> MKTMRKQIYKKAYWLLLPFLPLALANTFLVKEDSKNVTAYTPFATPITDSKSDLVSLAQLDSSYQIADQTIHNTNLFVLFKSRDVKVKYESSGSNNISFDSTSQGEKPSYVVEFTNSTNIGIKWTMVKKYQLDVPNVSSDMNQVLKNLILEQPLTKYTLNSSLAKEKGKTQREVHLGSGQANQWTSQRNQHDLNNNPSPNASTGFKLTTGNAYRKLSESWPIYEPIDGTKQGKGKDSSGWSSTEENEAKNDAPSVSGGGSSSGTFNKYLNTKQALESIGILFDDQTPRNVITQLYYASTSKLAVTNNHIVVMGNSFLPSMWYWVVERSAQENASNKPTWFANTNLDWGEDKQKQ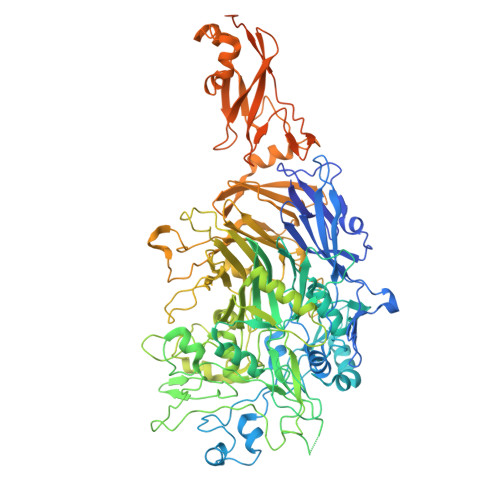FVENQLGYKETTSTNSHNFHSKSFTQPAYLISGIDSVNDQIIFSGFKAGSVGYDSSSSSSSSSSSSTKDQALAWSTTTSLDSKTGYKDLVTNDTGLNGPINGSFSIQDTFSFVVPYSGNHTNNGTTGPIKTAYPVKKDQKSTVKINSLINATPLNSYGDEGIGVFDALGLNYNFKSNQERLPSRTDQIFVYGIVSPNELRSAKSSADSTGSDTKVNWSNTQSRYLPVPYNYSEGIIDADGFKRPENRGASVTTFSGLKSIAPDGFANSIANFSVGLKAGIDPNPVMSGKKANYGAVVLTRGGVVRLNFNPGNDSLLSTTDNNIAPISFSFTPFTAAESAVDLTTFKEVTYNQESGLWSYIFDSSLKPSHDGKQTPVTDNMGFSVITVSRTGIELNQDQATTTLDVAPSALAVQSGIQSTTQTLTGVLPLSEEFSAVIAKDSDQNKIDIYKNNNGLFEIDTQLSNSVATNNGGLAPSYTENRVDAWGKVEFADNSVLQARNLVDKTVDEIINTPEILNSFFRFTPAFEDQKATLVATKQSDTSLSVSPRIQFLDGNFYDLNSTIAGVPLNIGFPSRVFAGFAALPAWVIPVSVGSSVGILFILLVLGLGIGIPMYRVRKLQDASFVNVFKKVDTLTTAVGSVYKKIITQTGVVKKAPSALKAANPSVKKPAAFLKPPVQPPSKPEGEQKAVEVKSEETKS>MKTVIQDTADVYFKRKSDGKLVFTAEAQTASFSQAISEEKLRGGIGNKPLYILKSEKEINLTVKNAFFDLEWLAMTQGETIQEETKVKVFDREHGLIVDDTNKVTLKGKPVSDVTFYNKKGLTYKIAVSTDGTYTIPTAFAAAKDKLTAVYQIEKVGRRLAIKASKFSERYEVEYRTIAYNPDTEEVYSDIYIQFPNVSPSGEFEMSLENGNALAPEIKFEALADTDTDEMAVVIEASRDENTAAPVEDTTGSTQSSDLGGTTE[2x];>MVKVDLESKRYGEKLKEVFLMLDNNVVECIKEITESSRNGKLVFFVGAGVSTLSDYPQWWRLVDKYHEELYGSPKKGNYSSDEYLRIPQIFYNVKGEMAFDGILKDFFQVDKPTNPIHDKILAMNPAHVITTNYDNLIDTACWKRGKYFSVISAEEDVANATSSRYLLKVHGDFRKGFKGENVVLKEDDYLNYDQNYPLISNLMKTIIATHTIVFIGYGLGDYNINMLLNWVRKLQKDSFHKPFFIRTDPSPIENETLIYYENKGLRIIDAASLIDSNEYDYLERYSAVMDLLIESQENKFITKDDEVIDYIYGKISPLFALQYIRKIDLKHVFEYDYHFEVNGTVVRHKNKGFGYMERFFELKESCDERSKLSKKQYERFNALFNFFEKNGVICMAKDAGTLNTSIEINSLAYHGKYDVMKKFIEEQSVSIEDDYKKAFFLACLGRWEESYDLYSNIILNSIDESNGCVYYLSQINRYRIYQSITQAVTQFNGLGLLTFGRHYKPFTDEFLARIEREMTNFNIDDLFNGMPFEFQKKYKILEFLSDNQFLYDDTVKLFELTNKVRSEMSEGSYSFGMSSDIVVLLRLYDNLRFLYENCLWSVSFHEFHQYIRNSMSLLIEKAEYERTRDIDELGFSFFGKKSGFFMEYYDFVNISRHFKIDDIKNLERSCSIDKIRFGEQEKIEEYLVGIAEEITKQFSANGMNVVFYTQFISEAKAALYFAKYVKLSEEGLGKIVKALLFYFPERDLDIGKRYVWLERLTKCNELPKSIISIIDDFLVLQAEKHIDQNYSEVSSNGLYSRDYGALIKHFEKNFISKRLSEITLCLTQDKQKQIDFLFKLLPLLSTNAKSHLLSFKSVENINDLMNGIRIGLIDEFTPEHEELIIEYLETRKVNYIVEKEKGIQTFSSNDYMSTFGIWYFLEEINNSKMEEFIGMDDQYDFFVDPENFDYKKFIPSWLKNYNDKLLGKIAGNKHMKHHVIEVLKERVKNSNDKRYLEILMNYFI[2x]

The defense-associated sirtuin 2 (DSR2) effector, a SIR2 domain-containing protein, protects bacteria from phage infection by depleting NAD+, while an anti-DSR2 protein (DSR anti-defense 1, DSAD1) is employed by some phages to evade this host defense. The NADase activity of DSR2 is unleashed by recognizing the phage tail tube protein (TTP). DSR2 is arranged as a dimer of dimers, which is facilitated by the tetramerization of SIR2 domains. DSR2 has a two-domain architecture, with the CTD responsible for sensing the infection signal and SIR2 acting to prevent phage propagation.

To elucidate the activation mechanism, we reconstituted the DSR2-TTP binary complex and analyzed its structure by cryo-EM. An elongated DSR2 tetramer binds four TTP molecules (termed state 1), each of which is nestled into a pocket primarily formed by H2-H4 subdomains and an additional H3 subdomain from the neighboring molecule. The outer sheet of the BS1 domain pairs with a stretch of residues (aa 903–910) in the H4 subdomain, while the inner sheet packs over the H3 subdomain. Specifically, A stretch of disordered region (aa 570–581) refolds into an ordered structure, including a β-strand, which interacts with the inner sheet of BS1 domain upon TTP binding, reminiscent of the observation in DSR2-DSAD1 complex. Two aromatic residues from the transition region, Tyr574 and Phe576, make hydrophobic and π-π stacking interactions with Ala9, Ala27, Ala30, Phe32 and Tyr175 from TTP. In addition, a loop segment (aa 493–504) of H2 transits into an α-helix in the presence of TTP. This α-helix of H2 subdomain fits snuggly into a pocket between the two slices of BS1, forming multiple hydrophobic contacts via Leu495, Leu497 and Leu498. Nonetheless, the inter-domain contacts between H2 and SIR2 appear to be weakened by the binding of TTP. Upon binding to TTP, the lid region shifts away from the active-site, possibly exposing the catalytic pocket for substrate binding. Mutation of the residues in the lid region responsible for inter-dimer association (Y71A/I90A and replacement of aa 78–96 with a GSAGSA linker) abrogated the NADase function of DSR2 in the presence of TTP, indicating that the lid region may modulate the catalytic activity of SIR2 domain. Together, it is reasonable to conclude that the TTP binding stimulates the rearrangement of the lid region, thereby activating the NADase function of the SIR2 domain.Tripartite ATP-independent periplasmic (TRAP) transporters are secondary transporters that have evolved an obligate dependence on a substrate-binding protein (SBP) to confer unidirectional transport. We investigated the significance of this interaction using the sialic acid-specific SBP, SiaP, from the Haemophilus influenzae virulence-related SiaPQM TRAP transporter. The first structure of a TRAP SBP revealed that the charge of the carboxylate group of the ligand, sialic acid, was neutralized by an arginine residue, Arg-147, in SiaP, which sequence analysis had revealed to be the most highly conserved residue, being present in 98% of TRAP SBPs of the common DctP family. Using in vitro, in vivo, and structural methods applied to SiaP, we demonstrate that the coordination of the acidic ligand moiety of sialic acid by the conserved arginine (Arg-147) is essential for the function of the transporter as a high affinity scavenging system.

To investigate whether this water network adds plasticity, i.e. ligand promiscuity, we engineered an R147E mutant to maintain the hydrophobic part of the arginine side chain and yet have the capacity to coordinate water 1 and water 3 observed in the R147A structure. In addition, by using the charge-swap from Arg to Glu, we can also assess the ability of the water molecules to dissipate the apparent charge clash. To investigate further the ability of the waters to relax the selectivity of SiaP for its ligands, the R147E mutant was crystallized in the presence of the non-cognate ligand sialylamide, which differs from Neu5Ac by a change of the carboxylate to an amide. The R147E-sialylamide co-crystal structure again reveals a closed conformation with an r.m.s.d. of 0.2 Å from the wild-type SiaP in complex with Neu5Ac. The amide and the opposing carboxylate group of Glu in the charge-swap mutant are linked by the two interstitial waters 1 and 3 in equivalent positions to those seen within the R147A mutant. The presence of the NH2 group results in the slight rearrangement of the water network around this ligand (waters 5–7 in Fig. 5A) as the NH2 group donates rather than accepts hydrogen bonds. In vivo data confirm the in silico predictions as growth of bacteria containing SiaP with the R147E mutation is more impeded than the R147K mutation but less than the R147A mutation. These data suggest that the two waters are able to accommodate two carboxylate groups pointing directly toward each other, while retaining sufficient function to enable bacterial growth. Our crystal structure confirmed that the mutant protein is able to use water-mediated contacts to bind sialylamide, an atypical ligand for SiaP. The finding that the wild-type protein was able to selectively bind this minor contaminating component, while R147E protein exposed to the same stock crystallized with the bound sialylamide, confirms the important role of the Arg-147 residue in the selectivity of SiaP for its cognate ligand.

> ADYDLKFGMNAGTSSNEYKAAEMFAKEVKEKSQGKIEISLYPSSQLGDDRAMLKQLKDGSLDFTFAESARFQLFYPEAAVFALPYVISNYNVAQKALFDTEFGKDLIKKMDKDLGVTLLSQAYNGTRQTTSNRAINSIADMKGLKLEVPNAATNLAYAKYVGASPTPMAFSEVYLALQTNAVDGQENPLAAVQAQKFYEVQKFLAMTNHILNDQLYLVSNETYKELPEDLQKVVKDAAENAAKYHTKLFVDGEKDLVTFFEKQGVKITHPDLVPFKESMKPYYAEFVKQTGQKGESALKQIEAINPHHHHHH1-methylindole-2,3-dione | C9 H7 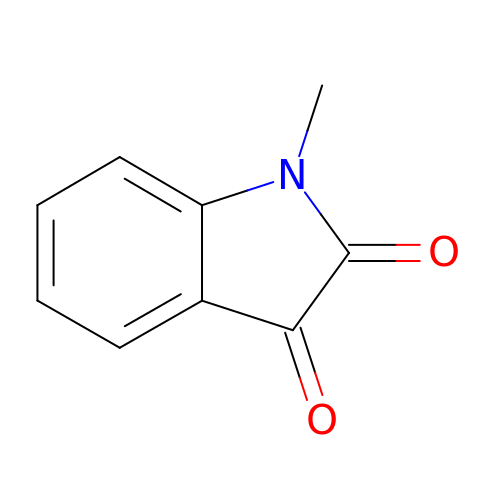N O2 | VCYBVWFTGAZHGH-UHFFFAOYSA-N α-2-Macroglobulins (α2Ms) are found in eukaryotic blood, invertebrate haemolymph, the eggs of birds and reptiles, and the bacterial periplasm, where they are thought to play a role in the restriction of proteolytic cleavage. Escherichia coli α2M (ECAM) contains the conserved thioester bond that is characteristic of the α2Ms and which is essential for covalent binding to cleaving proteases. Pbp1C is predicted to be a bifunctional transpeptidase and transglycosylase owing to its homology to Pbp1A and Pbp1B, which are both essential for the synthesis of the peptidoglycan layer. Both ECAM and Pbp1C are periplasmic proteins that are anchored to the inner membrane and have been proposed to function together in defence and repair against proteases that damage the bacterial cell wall. The overall structure of α2Ms comprises a series of β-sheet sandwich macroglobulin (MG) domains forming a ‘keyring’ shape, a bait-region domain (BRD) spanning the body of the ring, a mostly helical thioester domain (TED) connected to the ‘keyring’ by a complement protein subcomponent (CUB) domain, and a C-terminal MG (CTMG) domain.

To elucidate the mechanism of protease-induced α2M activation, we crystallized and solved the X-ray structure of a porcine elastase-cleaved form of ECAM, a close homologue of SaA2M (81% amino-acid sequence identity) for which the structure of the unactivated form was recently solved. However, an alternative strategy of in situ proteolysis and crystallization with selenomethionine-labelled ECAM was successful. This method yielded crystals that diffracted to 3.65 Å resolution. Analysis of elastase-cleaved ECAM by SDS–PAGE and mass spectrometry confirms that MG domains 1, 2, 3 and 7 are absent from the crystallized protein. Most notably, in the structure of the protease-cleaved ECAM, interactions between the TED and the CTMG domain, which protects the thioester bond in unactivated SaA2M, are not present. Thioester bond release is achieved by the untethering of a large region of an unstructured polypeptide chain upon cleavage of the BRD that forms new interactions with the CTMG domain, thereby preventing the protective interaction with the TED. Specifically, in the elastase-cleaved form of ECAM additional residues (Phe947–Asn963) of the BRD are observed that are disordered in the uncleaved SaA2M structure. The buried surface area between the CTMG domain and TED in SaA2M is 1972 Å2, with three hydrogen bonds between these domains, whereas the buried surface area between the elastase-cleaved BRD and the CTMG domain in ECAM is 1438 Å2, with five hydrogen bonds between the domains.

> NAPTAVKKDAPSEVTKAASSENASSAKLSVPERQKLAQQSAGKVLTLLDLSEVQLDGAATLVLTFSIPLDPDQDFSRVIHVVDKKSGKVDGAWELSDNLKELRLRHLEPKRDLIVTIGKEVKALNNATFSKDYEKTITTRDIQPSVGFASRGSLLPGKVVEGLPVMALNVNNVDVNFFRVKPESLPAFISQWEYRNPLANWQSDKLLQMADLVYTGRFDLNPARNTREKLLLPLGDIKPLQQAGVYLAVMNQAGRYDYSNPATLFTLSDIGVSAHRYHNRLDIFTQSLENGAAQQGIEVSLLNEKGQTLTQATSDAQGHVQLENDKNAALLLARKDGQTTLLDLKLPALDLAEFNIAGAPGYSKQFFMFGPRDLYRPGETVILNGLLRDADGKALPNQPIKLDVIKPDGQVLRSVVSQPENGLYHFTWPLDSNAATGMWHIRANTGDNQYRMWDFHVEDFMPERMALNLTGEKTPLTPKDEVKFSVVGYYLYGAPANGNTLQGQLFLRPLREAVSALPGFEFGDIAAENLSRTLDEVQLTLDDKGRGEVSTESQWKETHSPLQVIFQGSLLESGGRPVTRRAERAIWPADALPGIRPQFASKSVYDYRTDSTVKQPIVDEGSNAAFDIVYSDAQGVKKAVSGLQVRLIRERRDYYWNWSEDEGWQSQFDQKDLIENEQTLDLKADETGKVSFPVEWGAYRLEVKAPNEAVSSVRFWAGYSWQDNSDGSGAVRPDRVTLKLDKASYRPGDTIKLHIAAPTAGKGYAMVESSEGPLWWQEIDVRAQGLDLTIPVDKTWNRHDLYLSTLVVRPGDKSRSATPKRAVGVLHLPLGDENRRLDLALETPAKMRPNQPLTVKIKASTKNGEKPKQVNVLVSAVDSGVLNITDYVTPDPWQAFFGQKRYGADIYDIYGQVIEGQGRLAALRFGGDGDELKRGGKPPVNHVNIVVQQALPVTLNEQGEGSVTLPIGDFNGELRVMAQAWTADDFGSNESKVIVAAPVIAELNMPRFMASGDTSRLTLDITNLTDKPQKLNVALTASGLLELVSDSPAAVELAPGVRTTLFIPVRALPGYGDGEIQATISGLALPGETVADQHKQWKIGVRPAFPAQTVNYGTALQPGETWAIPADGLQNFSPVTLEGQLLLSGKPPLNIARYIKELKAYPYGCLEQTASGLFPSLYTNAAQLQALGIKGDSDEKRRASVDIGISRLLQMQRDNGGFALWDKNGDEEYWLTAYVMDFLVRAGEQGYSVPTDAINRGNERLLRYLQDPGMMSIPYADNLKASKFAVQSYAALVLARQQKAPLGALREIWEHRADAASGLPLLQLGVALKTMGDATRGEEAIALALKTPRNSDERIWLGDYGSSLRDNALMLSLLEENKLLPDEQYTLLNTLSQQAFGERWLSTQESNALFLAARTIQDLPGKWQAQTSFSAEQLTGEKAQNSNLNSDQLVTLQVSNSGDQPLWLRMDASGYPQSAPLPANNVLQIERHILGTDGKSKSLDSLRSGDLVLVWLQVKASNSVPDALVVDLLPAGLELENQNLANGSASLEQSGGEVQNLLNQMQQANIKHIEFRDDRFVAAVAVDEYQPVTLVYLARAVTPGTYQVPQPMVESMYVPQWRATGAAEDLLIVRPLEHHHHHH The initial enzyme in the degradation pathway is 3-nitrotoluene dioxygenase (3NTDO) which catalyses the oxidation of 3-nitrotoluene into a mixture of methylcatechols and nitrite. 3NTDO is a multicomponent enzyme system which adds two atoms of molecular oxygen to the substrate through the sequential action of three separate proteins. In this reaction, electrons originating from NADH/NADPH are transferred to FAD in the reductase, the first redox center which subsequently reduces the plant type [2Fe-2S] cluster in the reductase that, in turn, reduces the terminal oxygenase through a ferredoxin. 3NTDO from Diaphorobacter sp. strain DS2 belongs to the family of naphthalene dioxygenases, and has the ability to remove nitrite from all isomers of mononitrotoluene, 2-chloronitrobenzene, 2,6-dinitrotoluene and partially from 3-chloronitrobenzene.

3NTDO-ODS2 is a mushroom shaped hetero hexamer (α3β3) protein with a cap and a stem composed of the α3 and β3 subunits, respectively. The α-subunit contains Rieske domain (residues 38–158) with a Rieske [2Fe-2S] center and a catalytic domain (residues 1–37, 159–447) that contains a mononuclear iron at the active site. The completely conserved residues His206, His211 and Asp360 coordinate mononuclear iron. The tertiary and secondary structural elements as well as the essential residues in the electron transfer are conserved between 3NTDO-O and other known oxygenases. The structure has been refined to a final R value of 24% (Rfree = 28%) to 2.9Å resolution. All the residues except the three residues at the C-terminus of the α subunit could be located in the electron density map. The pocket size was found to be 445Å3(3NTDO), 295Å3(NBDO) and 693Å3 (NDO) respectively. This suggests that 3NTDO has a bigger pocket size than NBDO and this could explain the formation of other nitrophenol products–by facilitating binding of the larger substrate. Ile204, Met251, Asn258 and Val350 which line the pocket of the active site of 3NTDO, were mutated to corresponding residues of NDO (Ala206, Leu253, Val260 and Phe352). I204A/N258V mutation gave nitrobenzyl alcohol as a major product from all isomers of mononitrotoluene. These results suggest that, for nitrite release from mononitrotoluenes both Ile204 and Asn258 are equally important and their role is the proper anchoring of the substrate in 3NTDO.

>MSYQNLVSEAGLTQKHLIHGDKELFQHEMKTIFARNWLFLTHDSLIPSPGDYVTAKMGLDEVIVSRQNDGSVRAFLNVCRHRGKTIVHAEAGNAKGFVCNYHGWGYGTNGELQSVPFEKELYGDAIKKKCLGLKEVPRIESFHGFIYGCFDAEAPPLIDYLGDAAWYMEPTFKHSGGLELVGPPGKVVVKANWKTFAENFVGDIYHVGWTHASILRVGQSVFTPLAGNAMLPPEGSGLQMTSKYGSGMSLMWDYYAGNHSADLVPDLMAFGGAKQEKLAKEIGDVRARIYRSHLNGTIFPNNSFLTGSAAFKVWNPIDENTTEVWTYAFVEKDMPEDLKRRLADAVQRTVGPGGYWESDDNDNMETLSQNAKKYQSSNSDLIASLGFGKDVYGDECYPGVVGPSGASETSYRGFYRAYQAHISSSNWAEFENASRNWHTELTKTTD[3x];>[3x]MMINTQEDKLVSAHDAEEFHRFYIVQDDALLQEVNTLLTREAHLLDIQAYKAWLEHCVAPEIKYQVISRELRSTSERRYQLNDAVNIYNENYQQLKVRVEHQMDPQNWPNSPKIRFTRFVTNVTAAKDKSAPEMLHVRSNLILHRARRGNEVDVFYATREDKWKRIEGGGIQLVERFVDYPERILPHNLLVFL> GSPGISGGGGGILEASSLGAHHIHHFHGSSKHHSVPIAIYRSPASLRGGHAGTTYIFSKGGGQITYKWPPNDRPSTRADRLAIGFSTVQKEAVLVRVDSSSGLGDYLELHIHQGKIGVKFNVGTDDIAIEESNAIINDGKYHVVRFTRSGGNATLQVDSWPVIERYPAGRQLTIFNSQATIIIGGKEQGQPFQGQLSG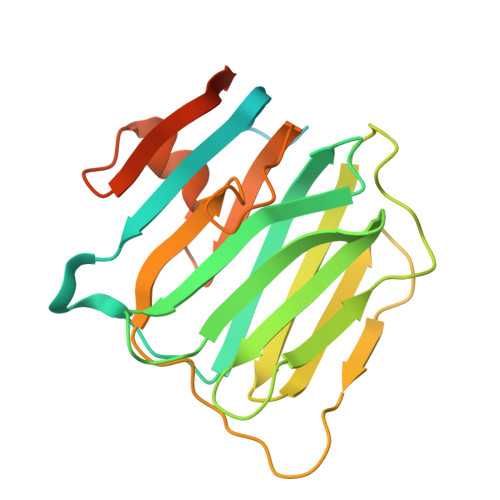LYYNGLKVLNMAAENDANIAIVGNVRLVGEVPSSMTTESHHHHHH> ELK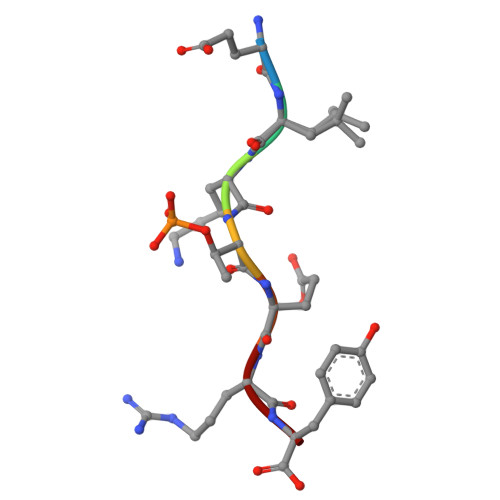TERY>[2x]SMGEIESYCNKELGPLPTKAPT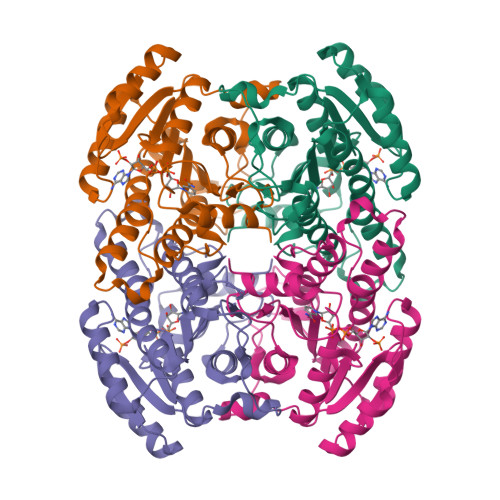LSKNVLDLFSLKGKVASVTGSSGGIGWAVAEAYAQAGADVAIWYNSHPADEKAEHLQKTYGVHSKAYKCNISDPKSVEETISQQEKDFGTIDVFVANAGVTWTQGPEIDVDNYDSWNKIISVDLNGVYYCSHNIGKIFKKNGKGSLIITSSISGKIVNIPQLQAPYNTAKAACTHLAKSLAIEWAPFARVNTISPGYIDTDITDFASKDMKAKWWQLTPLGREGLTQELVGGYLYLASNASTFTTGSDVVIDGGYTCP>[4x]GPSSPSLLRAIPGIAWIALLLLVIFYVFAVMGTKLFAQSFPEWFGTLGASMYTLFQ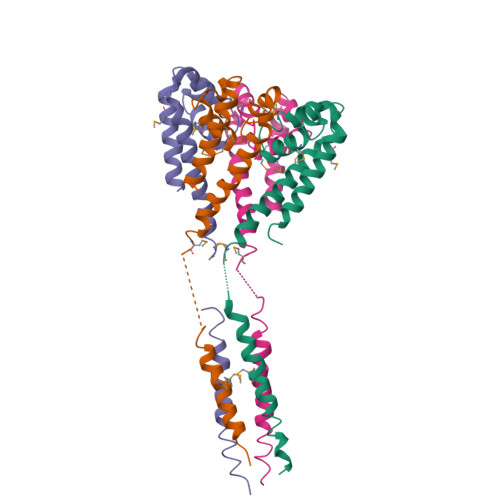VMTLESWSMGIARPVIEAYPWAWIYFVSFILVSSFTVLNLFIGIIIESMQSAHWEGGGAKRIEQEQRAHDERLEMLQLIRDLSSKVDRLERRSGKR> HTPVRTVMNTIQQLMMILNSASDQPSENLISYFNNCTVNPKESILKRVKDIGYIFKEKFAKAVGQGCVEIGSQRYKLGVRLYYRVMESMLKSEEERLSIQNFSKLLNDNIFHMSLLACALEVVMATYSRSTSQNLDSGTDLSFPWILNVLNLKAFDFYKVIESFIKAEGNLTREMIKHLERCEHRIMESLAWLSDSPLFDLIKQSKDREGPTDHLESA;> FQTQKPLKSTSLSLFYKKVYRLAYLRLNTLCERLLSEHPELEHIIWTLFQHTLQNEYELMRDRH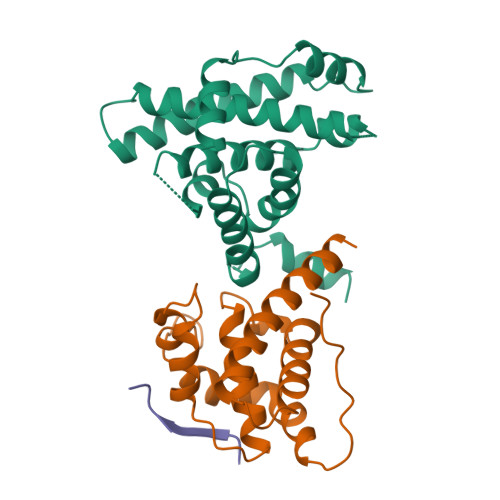LDQIMMCSMYGICKVKNIDLKFKIIVTAYKDLPHAVQETFKRVLIKEEEYDSIIVFYNSVFMQRLKTNILQYASTRPPTLSPIPHIPR;> DLYCYEQLN>[2x]LYFQGMDLTKQFPRSPVDRLGGMDHLKRVIDKARAHVAGTLGEYTYNCPLDQAFFSFFGLDHEKFAEAVKSRPQDQDMLAWVHSQSPRSKNPKEVESFN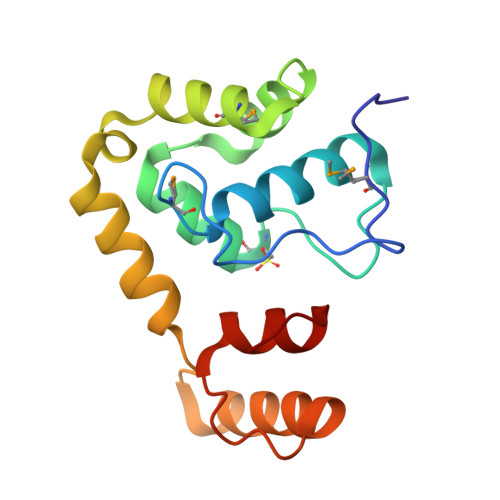REYESRSPDSPEKWDYFRSVRDSLAPGRTDITTWVKLLDLEEKRPV A new GlcNAc-specific lectin (PVL) was purified from the fruiting bodies and mycelium of a fungus, Psathyrella velutina and then structurally characterized. The PVL structure presents a novel fold among lectins, with seven β-sheets arranged in a β-propeller fold. The lectin therefore adopts a donut shape with six GlcNAc binding sites, and is expected to present strong avidity for cell surfaces presenting high density of terminal GlcNAc residues.

GlcNAc is also present in the branches of these glycoconjugates, either β1-2-linked to mannose (Man) on the trimannose core or β1-3-linked to galactose (Gal) as part of polylactosamine extended branches. Nevertheless, due to the activity of galactosyltransferases and sialyltransferases, these GlcNAc residues are not in terminal positions in normal tissues. Similarly glycosphingolipids contain GlcNAcβ1–3 or β1–6 linked to Gal but not in exposed terminal positions. The occurrence of aberrant βGlcNAc-terminating epitopes has been observed in a limited number of cancers, including human leukemia cells. The aim of the present work was to produce a recombinant form of PVL and to characterize its fine specificity towards the different GlcNAc-terminated epitopes that could be present on pathology-related truncated forms of human glycoconjugates. The avidity of the lectin for GlcNAc-decorated surface was evaluated on arrays. Finally, the ability of the lectin to label cancer cells and carcinoma tissues was also described.

>[2x]SVVVISQALPVPTRIPGVADLVGFGNGGVYIIRNSLLIQVVKVINNFGYDAGGWRVEKHVRLLADTTGDNQPDVVGFGENGVWISTNNGNNTFVDPPKMVLANFAYAAGGWRVEKHIRFMADLRKTGRADIVGFGDGGIYISRNNGGGQFAPAQLALNNFGYAQGWRLDRHLRFLADVTGDGLLDVVGFGENQVYIARNSGNGTFQPAQAVVNNFCIGAGGWTISAHPRVVADLTGDRKADILGFGVAGVYTSLNNGNGTFGAVNLVLKDFGVNSGWRVEKHVRCVSSLTNKKVGDIIGFGDAGVYVALNNGNGTFGPVKRVIDNFGYNQGWRVDKHPRFVVDLTGDGCADIVGFGENSVWACMNKGDGTFGPIMQLIDDMTVSKGWTLQKTVRYAANLYL1-{[3-(4-{[(2R)-4-(5-fluoro-2-methoxyphenyl)-2-hydroxy-4-methyl-2-(trifluoromethyl)pentyl]amino}-6-methyl-1H-indazol-1-yl)phenyl]carbonyl}-D-prolinamide 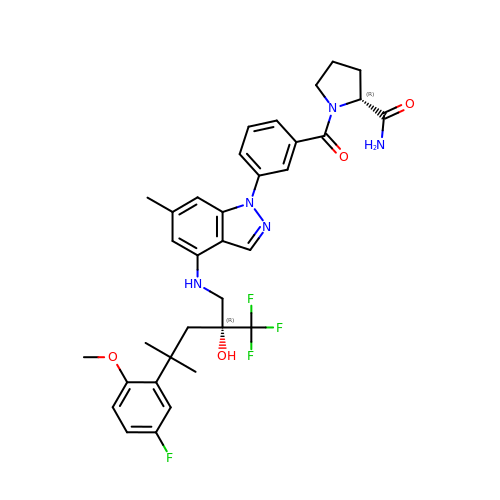| C34 H37 F4 N5 O4 | AKJCJJOQRAGWOW-ZORMNXRFSA-N>[3x]ILDGPYQPTTFTPPTDYWILINSNTNGVVYESTNNSDFWTAVIAVEPHVNPVDRQYNVFGENKQFNVRNDSDKWKFLEMFRGSSQNDFYNRRTLTSDTRLVGILKYGGRIW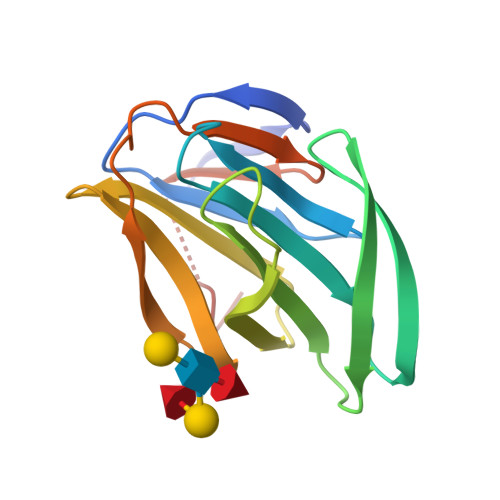TFHGETPRATTDSSNTANLNGISITIHSEFYIIPRSQESKCNEYINNGL>[2x]MQNTAKNAIWQRVRHSAIALSALSLFFGLQASELPQIPPQQVNNTMYQAFYWDAYPGLWANLPAMAAPLAERGITSMWLPPAAKGMNGTFSVGYDVYDLWDLGEFNQKGTTATRYGTRQQLQQALSALDQLGIQAYFDVVFNHRMGADAQEHIPGFGLAWTEYHLQGRQAHYTQQNWGYLWH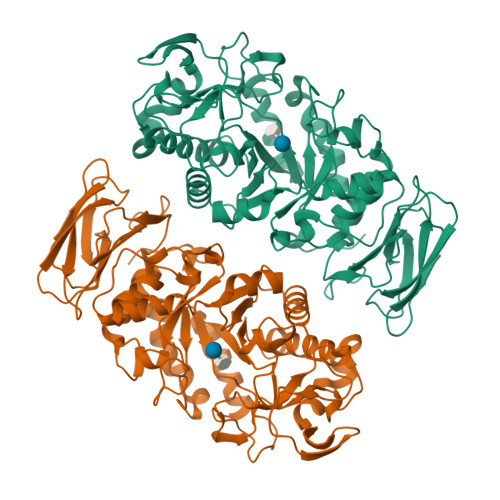DFDWNWTAFNGSDNQLYPGKWWGNTFHFPYLMGEDVDYNRFEVQQEMKAWGEWIINSVGFSGFRMDAIAHVDTDFTRDWINHVQWATSEDVFFVAEAWVSDINGYLDAVNTPHLRAFDFNLREDFVALSSGSKDMRWWGGLVNSQHRDRAVTFVDNHDTSRAGNPYGMPQVINYKNQAYAYILLREHGVPTVFARDYDEFGMAPTLDKLIEARRYFAYGPGHEYSGNTEAVYAYVREGLSTVPGTGLVMLISGRNWGGQQSFTINSHQPNTTFYDYTGNVSGTVTTNAQGYGSFPVTMTESTGWSVWVPQSNGGTQ1-[4-ethyl-5-[4-[(5-ethyl-1,2,4-oxadiazol-3-yl)methyl]piperazin-1-yl]carbonyl-2-methyl-1~{H}-pyrrol-3-yl]ethanone 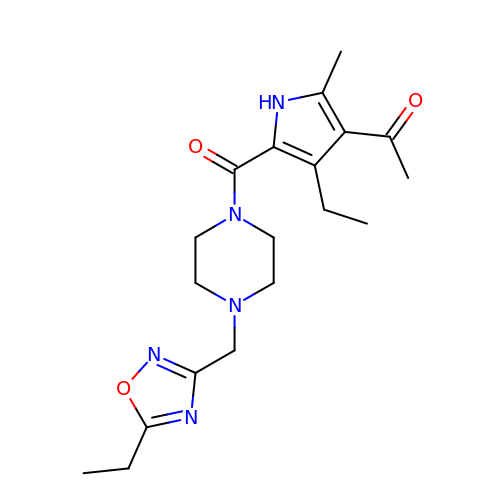| C19 H27 N5 O3 | AFYXSOFFFMWOFB-UHFFFAOYSA-N> VHHPPSYVAHLASDFGVRVFQQVAQASKDRNVVFSPYGVASVLAMLQLTTGGETQQQIQAAMGFKIDDKGMAPALRHLYKELMGPWNKDEISTTDAIFVQRDLKLVQGFMPHFFRLFRSTVKQVDFSEVERARF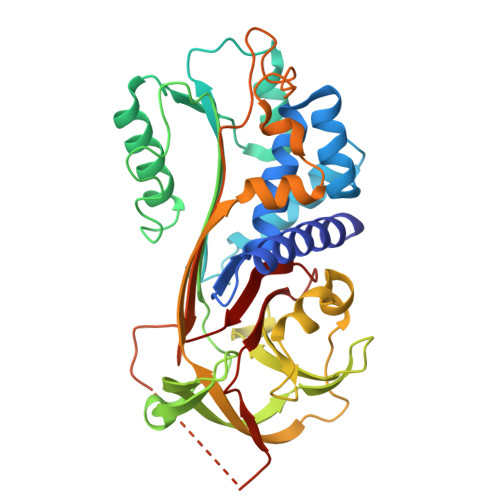IINDWVKTHTKGMISHLLGTGAVDQLTRLVLVNALYFNGQWKTPFPDSSTHRRLFHKSDGSTVSVPMMAQTNKFNYTEFTTPDGHYYDILELPYHGDTLSMFIAAPYEKEVPLSALTNILSAQLISHWKGNMTRLPRLLVLPKFSLETEVDLRKPLENLGMTDMFRQFQADFTSLSDQEPLHVALALQKVKIEVNESGTVASSSTAVIVSARMAPEEIIIDRPFLFVVRHNPTGTVLFMGQVMEP>[2x]SMRRTLGMQVRYVHHEDYQFCYSFRGRPGHKPSILMLHGFSAHKDMWLSVVKFLPKNLHLVCVDMPGHEGTTRSSLDDLSIDGQVKRIHQFVECLKLNKKPFHLVGTAMGGQVAGVYAAYYPSDVSSLCLVCPAGLQYSTDNQFVQRLKELQGSAAVEKIPLIPSTPEEMSEMLQLCSYVRFKVPQQILQGLVDVRIPHNNFYRKLFLEIVSEKSRYSLHQNMDKIKVPTQIIWGK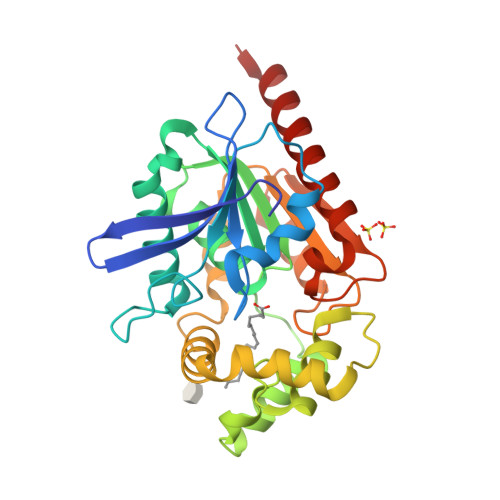QDQVLDVSGADMLAKSIANCQVELLENCGHSVVMERPRKTAKLIIDFLASVHNTDNNKKLD~{N}-[(~{E})-3-[(2~{R},3~{S},4~{R},5~{R})-5-(6-aminopurin-9-yl)-3,4-bis(oxidanyl)oxolan-2-yl]prop-2-enyl]-5-[(4-methylphenyl)methyl]-2,3-bis(oxidanyl)benzamide | C27 H28 N6 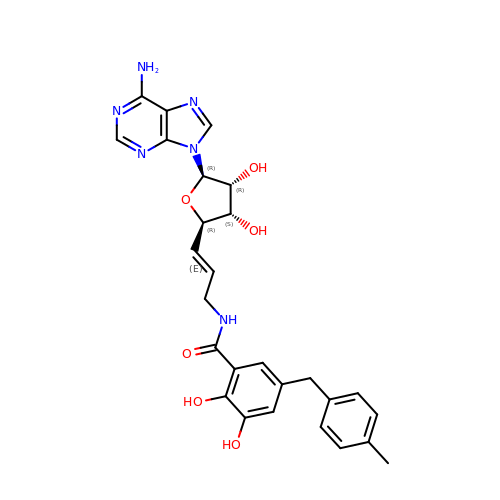O6 | FFSCJXJCNPYSCS-ZQIFPUEYSA-N>MGSSHHHHHHSSGLVPRGSMAEKFESRGIEEASSEVPTQRRCGAMEVHHRLLRSASYVRERDQIENLALKYKQGFRAISRMEIVKIPVVVHVVWNEEEENISDAQIQSQIDILNKDFRKLNSDVSQVPSVWSNLIADLGIEFFLATKDPNGNQTTGITRTQTSVTFFTTSDEVKFASSGGEDAWPADRYLNIWVCHVLKSEIGQDILGYAQFPGGPAETDGVVIVDAAFGTTGTALPPFDKGRTATHEI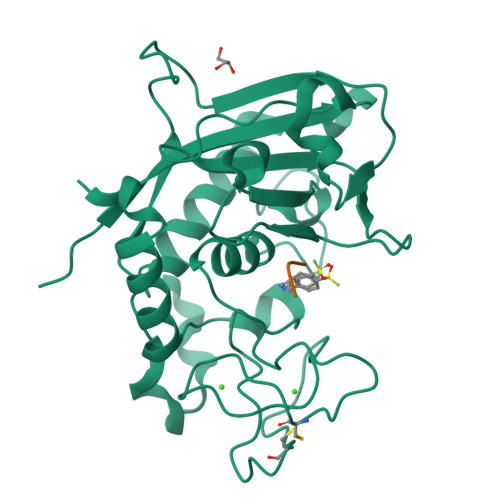GHWLNLYHIWGDELRFEDPCSRSDEVDDTPNQADPNFGAPSYPHVSCSNGPNGDMFMNYMDYVDDKCMVMFTQGQATRVNACLDGPRSSFLARVEETEKKEAPSKREMPMPR[2x];>[2x]GSS D-galacturonic acid | C6 H10 O7 | 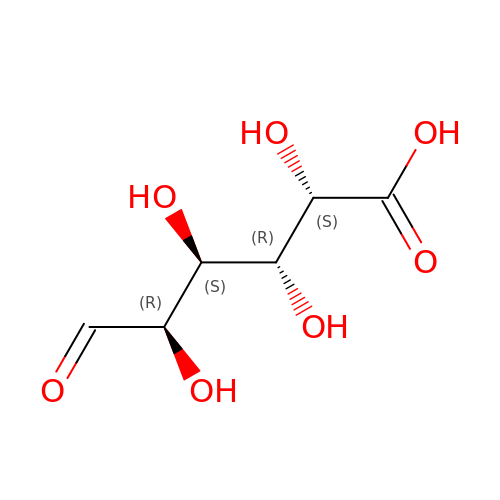IAJILQKETJEXLJ-RSJOWCBRSA-N Bacterial periplasmic binding proteins (PBP) are receptors for extracellular solutes in metabolite uptake, chemotaxis, and intercellular communication processes. The PBPs collectively constitute a structural protein superfamily characterized by two pseudo-symmetric domains that are linked by a hinge formed by two or three β-strands connecting the domains; a ligand-binding site is situated at the interface between the two domains. Solute binding induces a conformational change to form a closed state in which the ligand is bound at the domain interface and buried by the surrounding protein. We have characterized the stability, determined the ligand-binding properties, and solved the X-ray crystal structures of the apo and ligand-bound forms of a thermophilic periplasmic ribose-binding protein from the hyperthermophile Thermotoga maritima (tmRBP), the mesophilic homolog, ecRBP, of which has been studied in detail.

Crystals of ribose-complexed tmRBP were grown using a full-length wild-type construct (residues 30–323) that lacks the periplasmic signal sequence (residues 1–29). The X-ray crystal structure of ribose-bound tmRBP was solved by molecular replacement using ecRBP as the search model. The structure of the tmRBP ribose-complex is similar to the ribose complexes observed in ecRBP and a thermophilic RBP obtained from Thermoanaerobacter tengcongensis (tteRBP). The largest differences between ecRBP and tmRBP are at the C-termini, where tmRBP is extended by an additional 13 residues that are not present in ecRBP. Although ribose is commonly found as a furanose carbohydrate in biological molecules (e.g. nucleic acids), all periplasmic RBPs, including tmRBP, bind the β-anomer of D-pyranose ribose (as initially postulated by Koshland). β-D-pyranose ribose the most prevalent form in solution under ambient conditions (59%). The ligand-binding site of tmRBP is composed of a network of polar amino acids which is identical in sequence and hydrogen-bonding pattern to the E. coli protein. Seven polar amino acids make a total of eleven hydrogen-bonds with the ribose. The ribose is wedged between three aromatic amino acids (W15, F16 and F172) which make extensive van der Waals interactions with the sugar ring. The addition of ribose to tmRBP induces a 28° hinge-bending motion mediated about residues 102–105, 244–249, and 271–275. The amino acids in the N-terminal domain of the tmRBP binding pocket undergo large χ1 and χ2 torsional changes, whereas the C-terminal domain remains fixed.

> MKGKMAIVISTLNNPWFVVLAETAKQRAEQLGYEATIFDSQNDTAKESAHFDAIIAAGYDAIIFNPTDADGSIANVKRAKEAGIPVFCVDRGINARGLAVAQIYSDNYYGGVLMGEYFVKFLKEKYPDAKEIPYAELLGILSAQPTWDRSNGFHSVVDQYPEFKMVAQQSAEFDRDTAYKVTEQILQAHPEIKAIWCGNDAMALGAMKACEAAGRTDIYIFGFDGAEDVINAIKEGKQIVATIMQFPKLMARLAVEWADQYLRGERSFPEIVPVTVELVTRENIDKYTAYGRKEEGSHHHHHH>MSGSHHHHHHSGSMSERPSDLVVNRLVLFVVKGTATSTHNTVKPLILLEELGVPHDIYVVEKVSAPWFSEINPHKMVPAILDRSPDGRDTLRAWESTSTLMYIADAYDKDGTFGGRNVQERSEINNWLTLHTAALGPTARYWLYFYKLHPEKL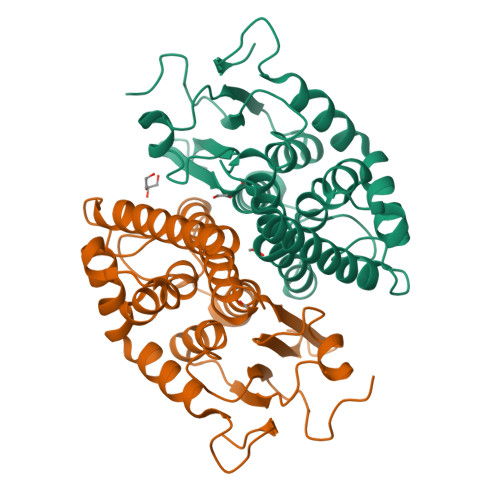PKTIEKLRSNITVQYDILERRLNEPGQQYLALKDRPTIADIATLPFAMKSTAELFGLEFEKWPKLQEWSVRMGEREAVKRAWQRVAGFGHGEKEYGMLEA[6x]>[3x]GSHMRLNLGGAEVFLRAEGLEEAPGGVRLWGREVRVFPPFPAKGFFRHGWQSWSLAAWVDPAQAPTPLLPEARRPQADDPFLLEAGAWWGSGVGALRGPDGRALLLGALDLGARVL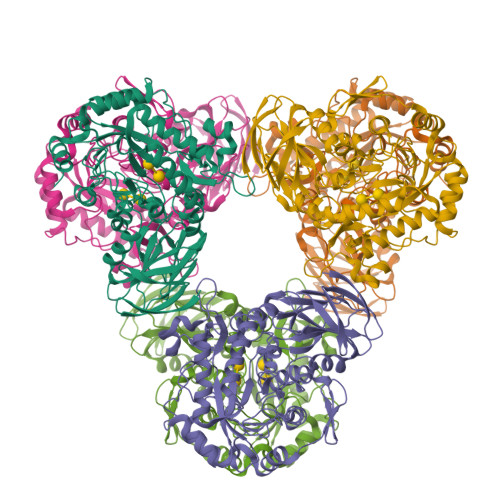GREDLLLGRYAGKGGAWFLAYGPEEEVFAAYARLLPRRLSGRPPRVWCSWYSFYTRIGEDLLLRVLDEVAAFSFEVFQIDDGWQRALGDWEPNDRFPRGMAFLAERIRERGLRAGLWFAPFLVTADSPLFQKRPDWVLRDGEGRPVRAGFNWGRPLYALDAGNEEVVEWAADLVRKALAWGYDYLKLDFLYAAALPGAEGEARYRKAMARLREAAGEAYLLFCGAPVLASLGLADGLRVGPDVAPYWDNEERSFWLADPTGPGLRNALRSTLHRLWLMENVHVDPDVVYFRTRFNLLSPEEMRLQEALAHFTGFKATSDPPSWLLPEEKGRLEAFLAREVPVRRLGPYRFRVGEEEVDYAPLL>MDVSFRLSGATSSSYGVFISNLRKALPNERKLYDIPLLRSSLPGSQRYALIHLTNYADETISVAIDVTNVYIMGYRAGDTSYFFNEASATEAAKYVFKDAMRKVTLPYSGNYERLQTAAGKIRENIPLGLPALDSAITTLFYYNANSAASALMVLIQSTSEAARYKFIEQQIGKRVDKTFLPSLAIISLENSWSALSKQIQIASTNNGQFESPVVLINAQNQRVTITNVD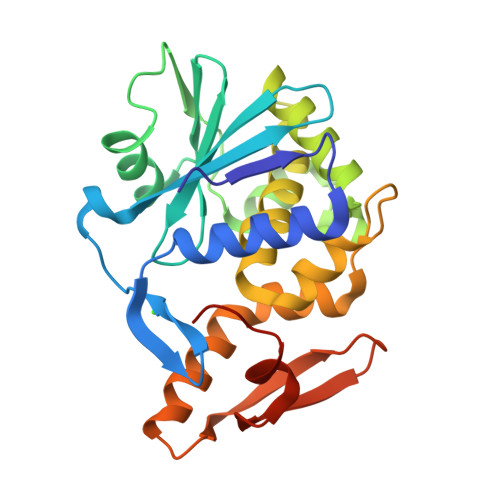AGVVTSNIALLLNRNNMA[4x]>[4x]GIDPFTMTPSEDFVVTDRGGIVENSHRVHAAVVDAKGRLLYALGNPTRMTLARSAAKPAQALAILETEGVAGYGFDDADIALMCASHSSEDRHIARTRAMLSKIKAEEADLRCGGHPSLSEMVNRSWIKQDFIPTAVCSNCSGKHVGMLAGARAIGAGTDGYHLPDHPMQGRVKRTVAELCDLDAGDVEWGTDGCNLPTPAFPLDRLGRIYAKLASAADGSDAGEGQSTRCAALAHIFRAMARHPEMVAGEGRYCTMLMRAFDGALVGKLGADASYAIGVRASDATRQLGTDGALGISVKIEDGNLEMLYAVVTELLERLGIGSPDVRSQLASFHHPQRVNTMGVTTGGVSFPFKLRGSKSNVDDPRLAAVAR

Rhizobium etli, a nitrogen-fixing bacterial symbiont of legume plants, encodes an essential l-asparaginase (ReAV) with no sequence homology to known enzymes with this activity. High-resolution crystal structures of ReAV show indeed a structurally distinct, dimeric enzyme, with some resemblance to glutaminases and β-lactamases. The active site of ReAV, deduced from structural comparisons and confirmed by mutagenesis experiments, contains a highly specific Zn2+ binding site without a catalytic role. There are two Ser-Lys tandems, all connected through a network of H-bonds to the Zn center, and three tightly bound water molecules near Ser48, which clearly indicate the catalytic nucleophile.

The orthorhombic (OP) and monoclinic MP1/MP2 forms show similar packing pattern with solvent content of 49.4–52.6%, whereas the monoclinic form MC, with a significantly different arrangement of the dimers in the unit cell, has 53.2% solvent content. In the close vicinity of the Ser48 hydroxyl, there is a characteristic, almost tetrahedral pattern of three closely-spaced water molecules w2, w3, w4, visible in all crystal structures, except MP2. On the other hand, Ser48 is not always hydrated (structure MP2) or the hydration may be incomplete and even different in the same crystal structure (triclinic crystals, not included in this study). In structure MP2, the side chain of Ser48 has two conformations: one as in the hydrated state but with H-bonds to w1, Lys51, Ser80 and another water molecule (different from w2/w3/w4). The second conformer of Ser48 is rotated ~110° and H-bonded to the N atom of Ala266 and carbonyl oxygen of Leu264. Except for the absence of the w2-w3-w4 water triad, no other structural rearrangements are observed in the vicinity of Ser48. The different hydration state might be the effect of differences in crystal vitrification prior to X-ray data collection. However, in our numerous collection of ReAV structures, we also see cases with incomplete or absent (MP2) water triad. The corresponding crystals were grown at different pH, detergent and salt conditions, which would certainly affect the protonation state of the key lysine residues and, therefore, polarization of Ser48. It can be hypothesized that in the crystal structure with no w2-w3-w4 triad and with double conformation of Ser48 (MP2), the hydroxyl group of Ser48 is not polarized and this structure shows the enzyme in its resting state, between catalytic cycles.> GAMEPLTASMLASAPPQEQKQMLGERLFPLIQAMHPTLAGKITGMLLEIDNSELLHML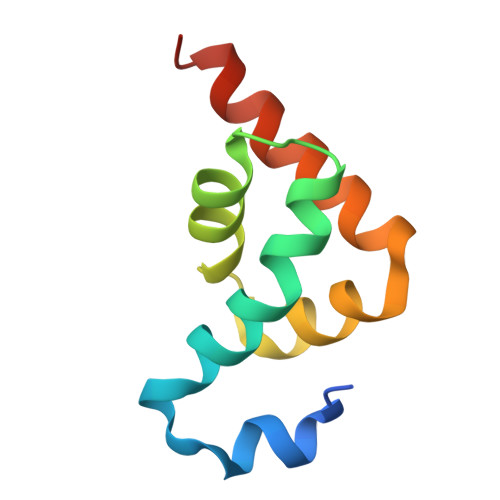ESPESLRSKVDEAVAVLQAHQAKE>[2x]MGSSHHHHHHSSGLVPRGSVCMTEIAT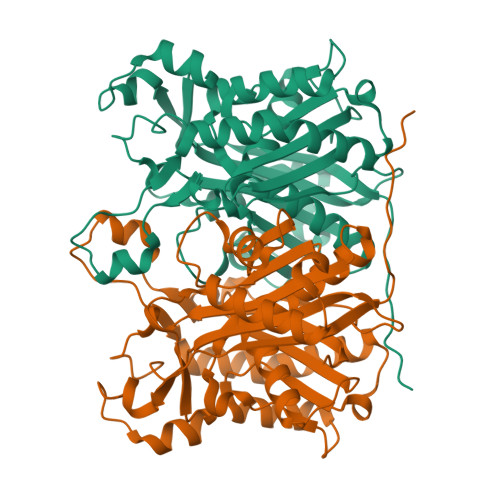TSGARSVGLLSVGAYRPERVVTNDEICQHIDSSDEWIYTATGIKTRRFAADDESAASMATEACRRALSNAGLSAADIDGVIVTTNTHFLQTPPAAPMVAASLGAKGILGFDLSAGCAGFGYALGAAADMIRGGGAATMLVVGTEKLSPTIDMYDAGNCFIFADGAAAVVVGETPFQGIGPTVAGSDGEQADAIRQDIDWITFAQNPSGPRPFVRLEGPAVFRWAAFKMGDVGRRAMDAAGVRPDQIDVFVPHQANSRINELLVKNLQLRPDAVVANDIEHTGNTSAASIPLAMAELLTTGAAKPGDLALLIGYGAGLSYAAQVVRMPKG>MGSMCPKDWKLFGSHCYLVPTVFSSASWNKSEENCSRMGAHLVVIHSQEEQDFITGILDI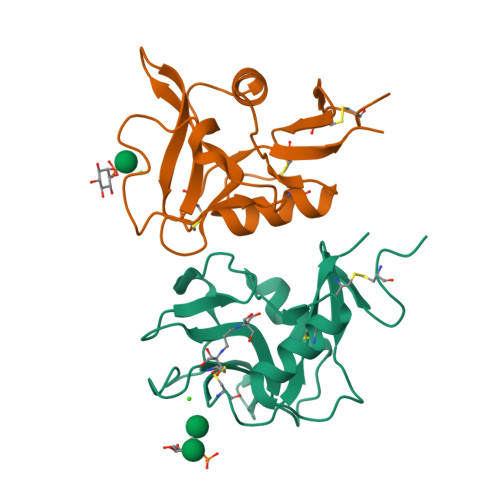HAAYFIGLWDTGHRQWQWVDQTPYEESVTFWHNGEPSSDNEKCVTVYYRRNIGWGWNDISCNLKQKSVCQMKKINL[2x]> GSHMEVNLRMSWWGGNGRHQVTLKALEEFHKQHPNINVKAEYTGWDGHLSRLTTQIAGGTEPDVMQT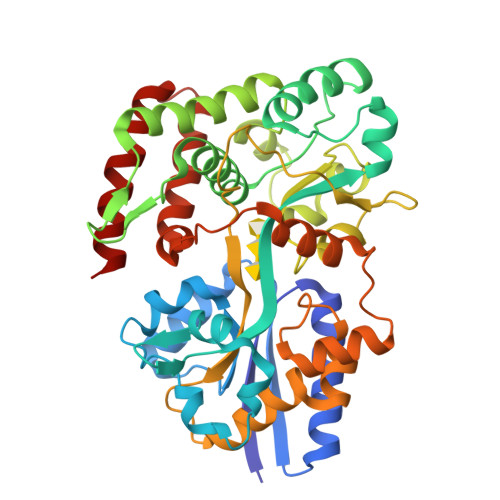NWNWLPIFSKDGTGFYNLFSVKEQLDLAQFDPKELQQTTVNGKLNGIPISVTARIFYFNDATWAKAGLEYPKTWDELLAAGKVFKEKLGDQYYPVVLEHQDTLALIRSYMTQKYNIPTIDEANKKFAYSPEQWVEFFTMYKTMVDNHVMPSTKYYASFGKSNMYEMKPWINGEWAGTYMWNSTITKYSDNLTKPAKLVLGPYPMLPGAKDAGLFFKPAQMLSIGKSTKHPQESAMLINFLLNSKEGVEALGLERGVPLSATAVTQLRASGVIKDEDPSVAGLNMALELPHKMTTSPYFDDPQIVSLFGDAIQYIDYGQKTVQETAEYFNKQGDRILKRAMR> ECPLSHDGYCLHDGVC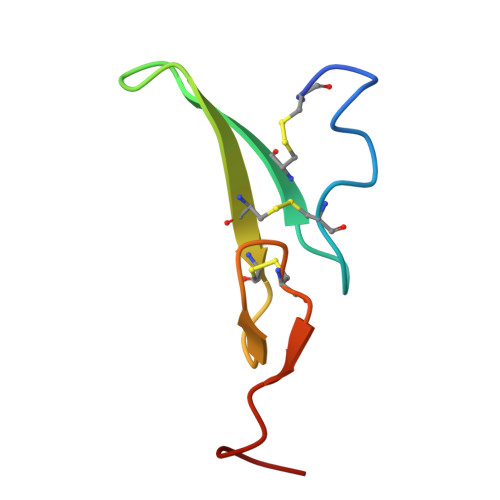MYIEALDKYACNCVVGYIGERCQYRDLKWWE> 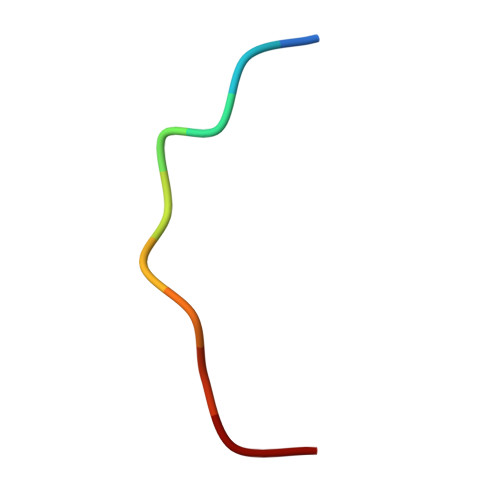GVVASQPARV Mitoguardin-2 (MIGA2), a mitochondrial outer membrane protein, forms the ERMCS in higher eukaryotic cells. Mammalian MIGA2 has several distinct domains: a mitochondrial targeting transmembrane domain (TM) at the N-terminus, a coiled-coil domain, the FFAT motif, and a large C-terminal LD targeting domain. Here, we report the crystal structures of the MIGA2 LD targeting domain and the major sperm protein (MSP) domain of VAPB bound to the phosphorylated FFAT motif of MIGA2. MIGA2 (yellow orange) forms a complex with VAPB (gray) via the phosphorylated FFAT motif and then transfers lipids between the membranes by extracting and interiorizing lipids into its large hydrophobic cavity.

We obtained crystals of the zebra fish Miga2 LD targeting domain (residues 310–568), which we refer to as zMiga2. zMiga2 shares 74.9% and 76.1% sequence identity to human and mouse LD targeting domains, respectively. A crystal of zMiga2 diffracted X-rays to 2.85 Å resolution, and the structure was solved by single-wavelength anomalous dispersion (SAD) using selenium as an anomalous scatterer. The zMiga2 structure resembles a “mug” and consists of eleven α-helices. The central six helices of the mug surround a large cavity of approximately 1100 Å3. Intriguingly, inside the cavity, we found extra electron density that seemed to correspond to that of a glycerophospholipid, although no glycerophospholipids were added during protein preparation or crystallization. We modeled this as PE with two 16:0 fatty acyl chains, since PE is the most abundant species in bacteria cells cultured in LB media. The central helices are amphiphilic with the hydrophobic sides facing inward; thus, the cavity is hydrophobic and can accommodate the hydrocarbon chains of a glycerophospholipid. Side chains of helices α3 (F370, M371, and M377), α6 (F426 and L431), α10 (I525 and Y528), and α11 (L561) make hydrophobic interactions with the first hydrocarbon chain. The hydrophobic side chains of helices α4 (Y396 and M399), α6 (I429 and I434), and α9 (F488, F492, I495, V499, and L503) contact the second hydrocarbon chain. Based on its structure, we found that zMiga2 has a positively charged concave surface in the handle region composed of helices α7 and α8.

> AGSLKPAALYEEALSLVKDGDVACRSLRTELLECYSDQDFLAKLHCVRQAFQVLLLDETHRMFFMETGKQMISGLLVKANKSPKAFLESYEDMLQYTQREETWPVSKMELEGRGVVCMNFFDIVLDFILMDAFEDLESPPSSVVAVLRNRWLSDSFKETALATACWSVLKAKRRLLMVPDGFIAHFYVISEHVSPVLAFGFLGPHQHLSEVCTIFKQQIVQYLKDMFDHDKVRFTSVPSLAEDILRLSHRRADILMGYLGIE> MAKDIEISASESKFILEALRQNYRLDGRSFDQFRDVEITFGKEFGDVSVKMGNTKVHCRISCQIAQPYEDRPFEGLFVISTEISPMAGSQFENGNITGEDEVLCSRIIEKSVRRSGALDVEGLCIVAGSKCWAVRADVHFLDCDGGFIDASCIAVMAGLMHFKKPDITVHGEQIIVHPVNEREPVP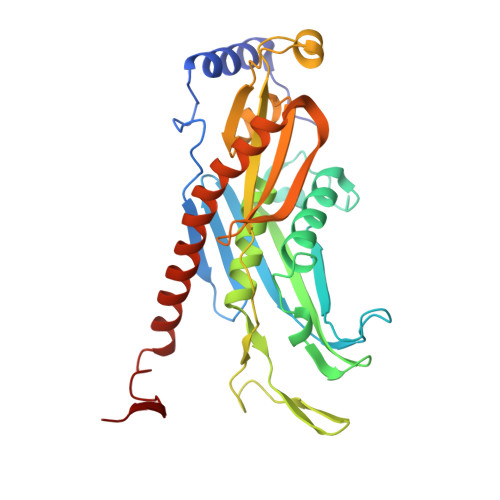LGILHIPICVTFSFFNPQDTEENIKGETNSEISIIDATLKEELLRDGVLTVTLNKNREVVQVSKAGGLPMDALTLMKCCHEAYSIIEKITDQILQLLKEDSEKRNKYAAMLTSENAREI> MKKLLIIGTGGTIASAKTEQGYKSVLKIDEILKLAKIKLENGYKIDSTNIMNIDSTLIHPEDWEIIAKEVFKALDDYDGIIITHGTDTLAYTASMLSFMIKNPNKPIVLTGSMLPITENGSDAPRNIRTAIKFAMEDVAGVFVAFMDKIMLGCRTSKVRTLGLNAFMSINYPDVAYVKGEKILYNIPKEKFQPNGSPELDTKYEPRVVVLRVTPGLGGEIIDAVLDAGYKGIVLEGYGAGGLPYRKSNLLSKIKEITPKIPVIMTTQALYDGVDMRKYEVGRKALETGIIPAKDMTKEATITKLMWALGHTKDVEKIREIMHTNYVNEIKS

The hyperthermophilic L-ASNase from Thermococcus sibiricus (TsAI) was previously shown to exhibit high activity and thermostability and is promising for biotechnology. L-ASNase exerts its anticancer activity by hydrolyzing L-asparagine (L-Asn) in the bloodstream to L-aspartic acid and ammonia. The subunit of TsAI consists of two α/β domains: an N-terminal large domain (residues 1–184, consisting of twelve mixed β-sheets and four α-helices) and a C-terminal small domain (residues 207–331, consisting of three β-sheets and five α-helices) connected by an interdomain linker (residues 185–206). In the N-terminal domain, the active site pocket of TsAI includes residuesthat are highly conserved among all types of L-ASNases: Y22, S55, T56, T86, D87, K157, and T12, which initiates the reaction.

The crystal structure of TsAI was solved at 1.9 Å. The asymmetric unit contained one copy of the protein. Crystal contact analysis showed that TsAI is a dimer in crystal as in solution. In the TsAI structure, T56 forms a water-mediated hydrogen bond with S15. The side chain of D54 forms a hydrogen bond network with G11, S55, and T56. The position of this loop is additionally fixed by the interaction of the side chain S55 with T9 and G85. The network of hydrogen bonds formed between D54 and G11, S55, and T56, along with the interaction of the side chain of S55 with T9 and G85, was shown to restrict loop motion in the wild-type enzyme. Thus, the higher rigidity of the loop M51-L57 is significant for maintaining increased thermostability of the native thermo-ASNase TsAI. In the wild-type enzyme, adaptive mutations stabilized the loop by a network of H-bonds and replaced the highly thermolabile glutamine residue with threonine to ensure proper function at elevated temperatures. Structural superposition of TsAI with TkA, PhA, PfA, EcAI, and EcAII (RMSD between TsAI and these structures are 0.5 Å, 0.6 Å, 0.5 Å, 1.5 Å, and 1.5 Å, respectively) revealed high conservation of the active site architecture and similarity in overall topology of non-catalytic regions, regardless of type, origin (taxonomy), and degree of sequence identity.> MS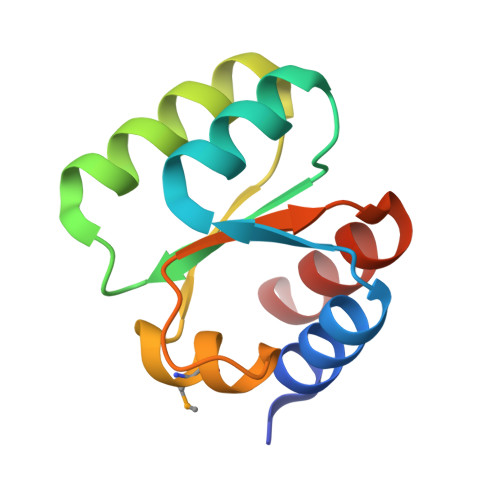EAKWLSLLGLAARARQLLTGEEQVVKAVQNGQVTLVILSSDAGIHTKKKLLDKCGSYQIPVKVVGNRQMLGRAIGKHERVVIGVKDAGFSRKLAALIDE>MENPLQKARILVNQLEKYLDRYAKEYDVEHLAGPQGHLVMHLYKHPDKDMSIKDAEEILHISKSVASNLVKRMEKNGFIAIVPSKTDKRVKYLYLTHLGKQKATQFEIF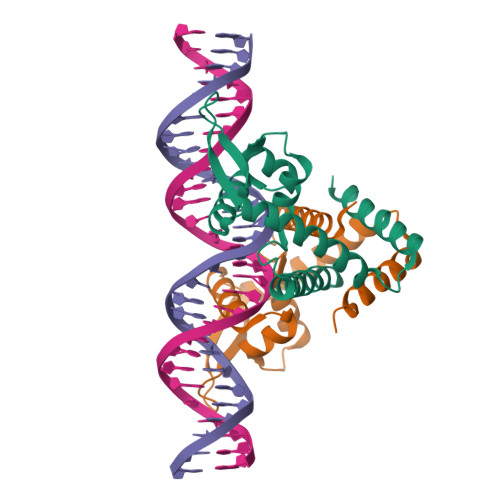LEKLHSTMLAGITKEEIRTTKKVIRTLAKNMAMEDFDSLEVLFQ[2x]>[4x]ELKPSRTVEKHIKTKYNLGNANYRIQ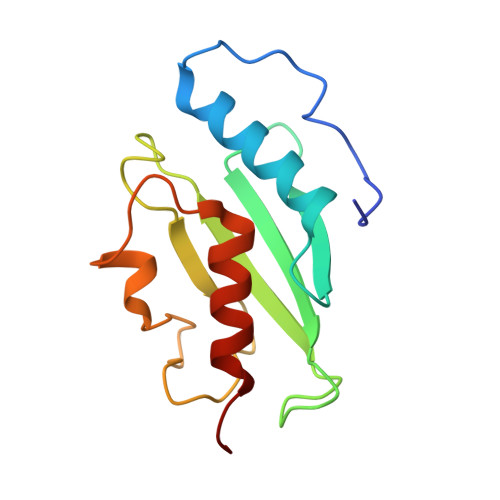KELNNFLKNPPINCTIDVHPSNIRIWIVQYVGLENTIYANEVYKIKIIFPDNYPLKPPIVYFLQKPPKHTHVYSNGDICLSVLGDDYNPSLSISGLILSIISMLSSAKEK>[24x]MASISEKMVEALNRQINAEIYSAYLYLSMASYFDSIGLKGFSNWMRVQWQEELMHAMKMFDFVSERGGRVKLYAVEEPPSEWDSPLAAFEHVYEHEVNVTKRIHELVEMAMQEKDFATYN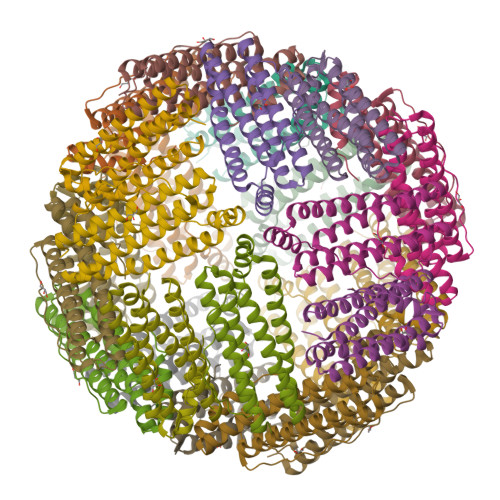FLQWYVAEQVEEEASALDIVEKLRLIGEDAAALLFLDKELSLRQFTPPAEEEK>AIKRIGNHITKSPEDKREYRGLELANGIKVLLISDPTTDKSSAALDVHIGSLSDPPNIAGLSHFLEHMLFLGTKKYPKENEYSQFLSEHAGSSNAFTSGEHTNYYFDVSHEHLEGALDRFAQFFLSPLFDESAKDREVNAVDSEHEKNVMNDAWRLFQLEKATGNPKHPFSKFGTGNKYTLETRPNQEGIDVRQELLKFHSAYYSSNLMAVVVLGRESLDDLTNLVVKLFSEVENKNVPLPEFPEHPFQEEHLKQLYKIVPIKDIRNLYVTFPIPDLQKYYKSNPGHYLGHLIGHEGPGSLLSELKSKGWVNTLVGGQKEGARGFMFFIINVDLTEEGLLHVEDIILHMFQYIQKLRAEGPQEWVFQELKDLNAVAFRFKDKERPRGYTSKIAGILHYYPLEEVLTAEYLLEEFRPDLIEMVLDKLRPENVRVAIVSKSFEGKTDRTEEWYGTQYKQEAIPDEVIKKWQNADLNGKFKLPTKNEFIPTNFEILPLEKEATPYPALIKDTAMSKLWFKQDDKFFLPKANLNFEFFSPFAYVDPLHSNMAYLYLELLKDSLNEYAYAAELAGLSYDLQNTIYGMYLSVKGYNDKQPILLKKIIEKMATFEIDEKRFEIIKEAYMRSLNNFRAEQPHQHAMYYLRLLMTEVAWTKDELKEALDDVTLPRLKAFIPQLLSRLHIEALLHGNITKQAALGIMQMVEDTLIEHAHTKP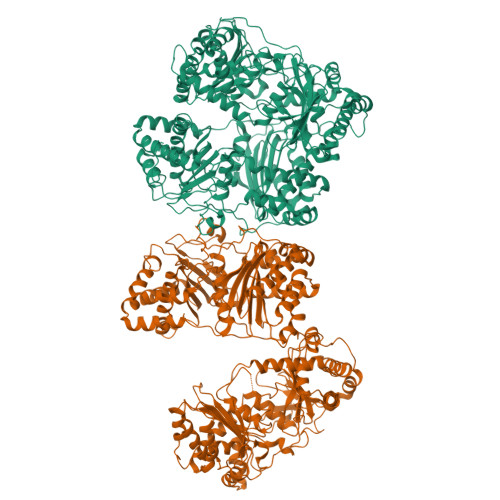LLPSQLVRYREVQLPDRGWFVYQQRNEVHNNSGIEIYYQTDMQSTSENMFLELFAQIISEPAFNTLRTKEQLGYIVFSGPRRANGIQGLRFIIQSEKPPHYLESRVEAFLITMEKSIEDMTEEAFQKHIQALAIRRLDKPKKLSAESAKYWGEIISQQYNFDRDNTEVAYLKTLTKEDIIKFYKEMLAVDAPRRHKVSVHVLAREMDSCPVVGEFPCQNDINLSQAPALPQPEVIQNMTEFKRGLPLFPLVKPH[2x]>MPLPTTLRPTLRQIRSELAAQLFDHILPFWLGQQDPIHGGFYGSITTGPDPTAPKGLVMTARHLWTFSQAFLSRPNPAYLEAAGNAYRFLTHALYDATHRGFFWSVHPDGTPLSRVKKLYGNAFAVYALAAYHTASGDREALTLAWETFDLLEDRGRDRRHGGYYEAFTEDWSTPLPEPLGEGETPAPKTMNTHLHILEAYSTLFRTTKEPRVREAMEHLILIFRTHIAPSSHLGLYFAEDWAPMGGGISFGHDIEATWL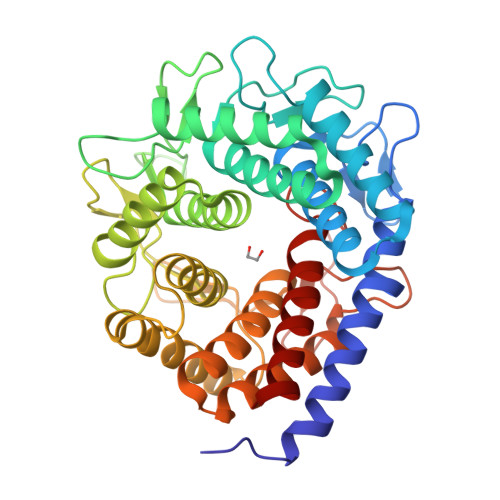LTESVELLYGDPLPEWFLSWIRPVMEETARALDTHGGSLPNEQREDGSVDRARVWWVQAEAFVGFLNAYSLFEEPRYLDHACTVWRFIMDHLVDREGGEWFWAVTPEGSPLAGYEKGGMWKASYHNSRACLEGMRRIDTILEEE[4x]>[3x]MSTAAKQNRSTSRVSKKKTAAPKEGAAKKSDKGHKYEYVELAKASLTSAQPQHFYAVVIDATFPYKTNQERYICSLKIVDPTLYLKQQKGAGDASDYATLVLYAKRFEDLPIIHRAGDIIRVHRATLRLYNGQRQFNANVFYSSSWALFSTDKRSVTQEINNQDAVSDTTPFSF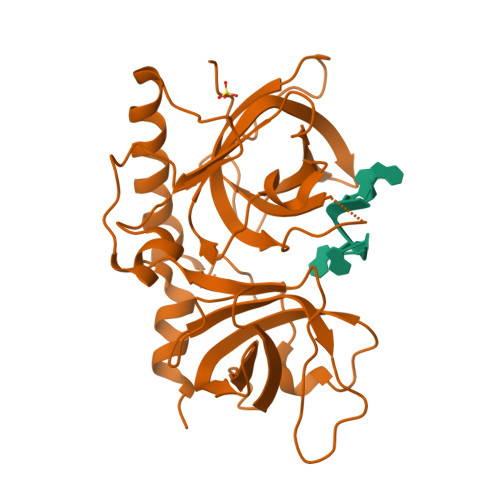SSKHATIEKNEISILQNLRKWANQYFSSYSVISSDMYTALNKAQAQKGDFDVVAKILQVHELDEYTNELKLKDASGQVFYTLSLKLKFPHVRTGEVVRIRSATYDETSTQKKVLILSHYSNIITFIQSSKLAKELRAKIQDDHSVE> ETG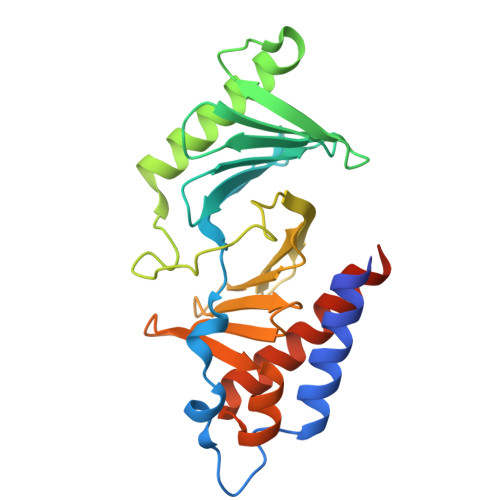EVVDCHLSDMLQQLHSVNASKPSERGLVRQEEAEDPACIPIFWVSKWVDYSDKYGLGYQLCDNSVGVLFNDSTRLILYNDGDSLQYIERDGTESYLTVSSHPNSLMKKITLLKYFRNYMSEHLLKAGANITPREGDELARLPYLRTWFRTRSAIILHLSNGSVQINFFQDHTKLILCPLMAAVTYIDEKRDFRTYRLSLLEEYGCCKELASRLRYARTMVDKLLSSRSASNRLKAS> QRCGEQGSNMECPNNLCCSQYGYCGMGGDYCGKGCQNGACWTSKRCGSQAGGATCTNNQCCSQYGYCGFGAEYCGAGCQGGPCRADIKCGSQAGGKLCPNNLCCSQWGFCGLGSEFCGGGCQSGACSTDKPCGKDAGGRVCTNNYCCSKWGSCGIGPGYCGA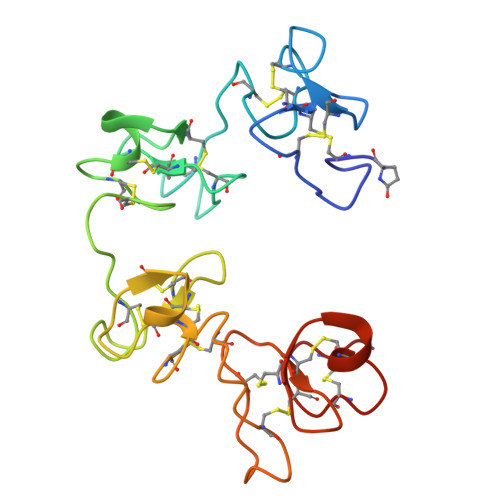GCQSGGCDG>[5x]MAQLTQMTNEQLRELIEAVRAAAVGAAGSAAAAGGADASRGKGNFSACTHSFGGTRDHDVVEEFIGNIETYKDVEGISDENALKGISLLFYGMASTWWQGVRKEATTWKEAIALIREHFSPTKPAYQIYMEFFQNKQDDHDPIDTFVIQKRALLAQLPSGRHDEETELDLLFGLLNIKYRKHISRHSVHTFKDLLEQGRIIEHNNQEDEEQLATAKNTRGSKRTTRCTYCSFRGHTFDNCRKRQKDRQEE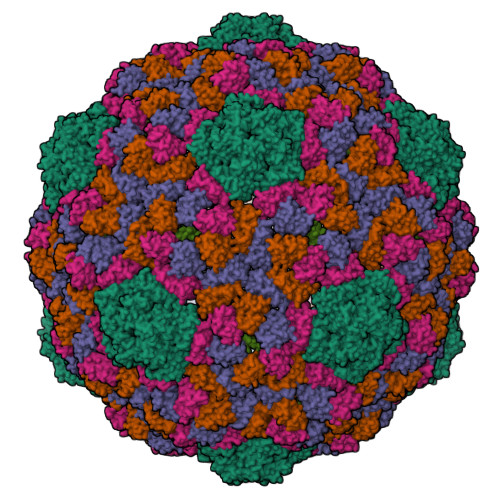QHEE> MGPREVTMKKGDILTLLNSTNKDWWKVEVNDRQGFVPAAYVKKLDSGTGKELVLALYDYQEK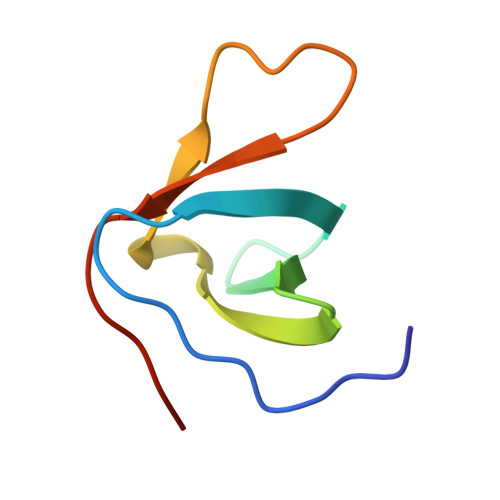S>[8x]SGCSTVDTVKDFNKDNFFTGSWYM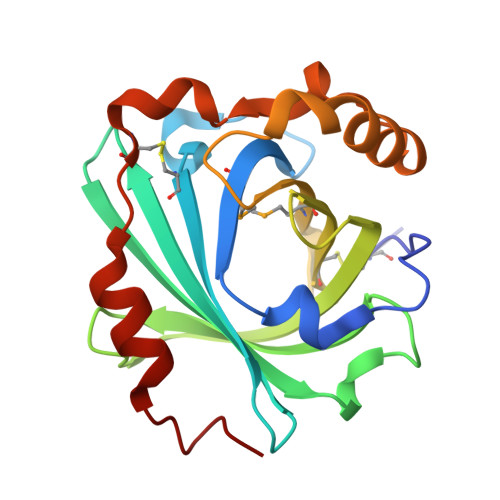THYKLGDSTLEVGDKNCTKFLHQKTADGKIKEVFSNYNPNAKTYSYDISFAKVSDFDGNNGKYTAKNVIVEKDGRKIDERTLQVSYIDTDYSKYSVVHVCDPAAPDYYMYAVQSRTENVKEDVKSKVEAALGKVGLKLSGLFDATTLGNKCQYDDETLQKLLKQSFPNYEK>[8x]DLILPFYKAGKVSFYQGDLDVLINFLEPDVLVNAANGDLRHVGGVARAIDVFTGGKLTKRSKEYLKSSKAIAPGNAVLFENVLEHLSVMNAVGPRNGDSRVEGKLCNVYKAIAKCDGKILTP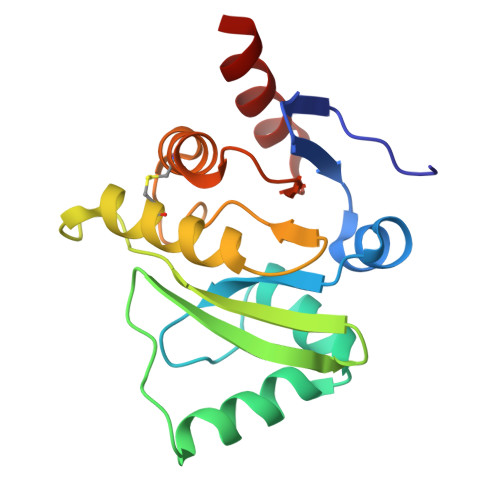LISVGIFKVKLEVSLQCLLKTVTDRDLNVFVYTDQERVTIENFFNG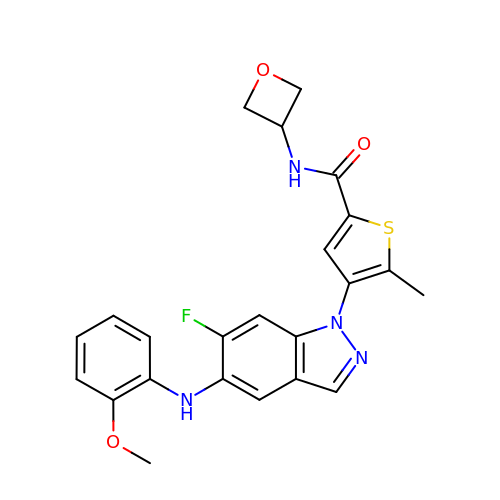(4P)-4-[6-fluoro-5-(2-methoxyanilino)-1H-indazol-1-yl]-5-methyl-N-(oxetan-3-yl)thiophene-2-carboxamide | C23 H21 F N4 O3 S | HCBJDOHJSNTYMP-UHFFFAOYSA-N(2R)-pentan-2-ol | C5 H12 O 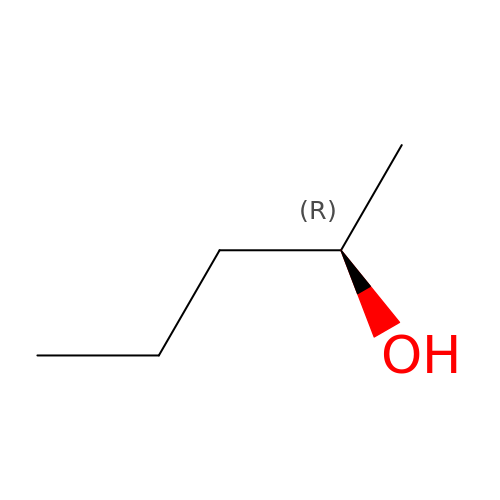| JYVLIDXNZAXMDK-RXMQYKEDSA-N>GPLGSLNDIEEIRFTARSEENLRGVHPDLVRVIRLALRYSLVPFSVSEGLRSMARQREMVRAGSSQTLRSRHLTGHAVDVVAMPAGVVSWEWDYYAQIAVAVRRAARECGIIVEWGGEWKTLKDGPHFQLTFRDYPA[2x]

The high-resolution crystal structure of S. marcescens ChiX reveals that the protein belongs to the lysostaphin-type, d-Ala d-Ala metallopeptidases and sonic hedgehog ‘LAS’ family of Zn2+-dependent peptidases. In vitro assays then establish ChiX as an l-Ala d-Glu endopeptidase that cleaves the cross-links in bacterial peptidoglycan, and site-directed mutagenesis is used to demonstrate that the chitinase secretion controlled by ChiX is directly attributable to this catalytic activity. A mutant strain of S. marcescens devoid of ChiX was found to be impaired in the secretion of a select subset of ∼10 proteins, including all known chitinases and chitin-binding proteins. Available evidence suggests that ChiX relies on its partner protein, the holin ChiW, to gain access to the periplasm and that this is the only role of the membrane-bound ChiW in chitinase secretion.

The asymmetric unit contains two ChiX molecules (labelled A and B), and the model for each consists of ChiX residues 2–134, with residue 1 (serine) originating from the genetic construct. ChiX presents an α/β-fold that consists of five α-helices, and four antiparallel β-strands are arranged as a single β-sheet in the order β1–β2–β4–β3. On the other side, and linking β1 and β2, α3 and a short α4 form a helical loop. This loop is orthogonal to the β-sheet, and together, they create an open and deep, mainly hydrophilic cleft. The Zn2+-binding site is at the base of this cleft and is primarily created by residues from one side of the β-sheet. The cation displays tetrahedral co-ordination geometry typical of many Zn2+-dependent enzymes involving two nitrogen and two oxygen atoms. Two histidines, His68 contributed from α4 and His123 from β4, co-ordinate the metal through NE2 and ND1, respectively. The third co-ordinating group is Asp75 OE1 and the fourth is provided by Glu7 OE2 from the N-terminal tail of another ChiX molecule (molecule B) in the asymmetric unit. However, while data presented in this study clearly demonstrate that ChiX Asp120 is critical for enzymatic activity, the structural alignment with Ply500 indicates that ChiX Asp120 is pushed away from the metal ion relative to the equivalent Asp130 in Ply500. Indeed, while the closest Asp to Zn2+ distance is 4.0 Å in Ply500, it extends to 7.3 Å in ChiX. This difference in conformation is potentially due to the salt bridge formed between Asp120 and Arg34 of the adjacent ChiX molecule in the asymmetric unit and further compounded by the presence of Glu7 also from the adjacent molecule, which forms the fourth co-ordination point with the Zn2+ and would prevent Asp120 moving closer due to electrostatic repulsion.> MPVITLPDGSQRHYDHAVSPMDVALDIGPGLAKACIAGRVNGELVDACDLIENDAQLSIITAKDEEGLEIIRHSCAHLLGHAIK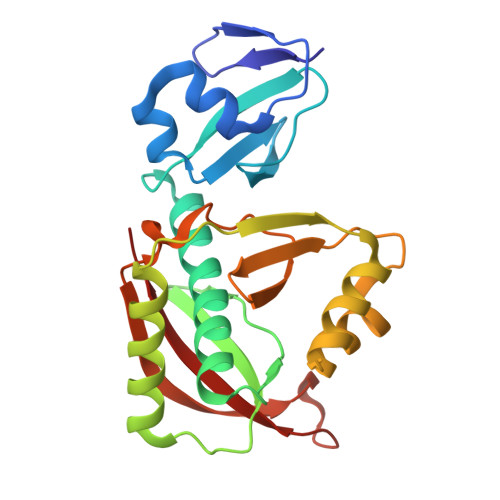QLWPHTKMAIGPVIDNGFYYDVDLDRTLTQEDVEALEKRMHELAEKNYDVIKKKVSWHEARETFANRGESYKVSILDENIAHDDKPGLYFHEEYVDMCRGPHVPNMRFCHHFKLMKTAGAYWRGDSNNKMLQRIYGTAWA4-[8-azanyl-3-[(2~{S})-1-[4-(dimethylamino)butanoyl]pyrrolidin-2-yl]imidazo[1,5-a]pyrazin-1-yl]-~{N}-(1,3-thiazol-2-yl)benzamide 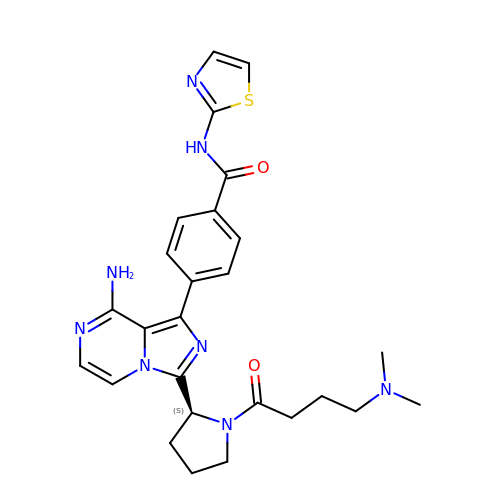| C26 H30 N8 O2 S | HUXVNVAKNWKLJM-IBGZPJMESA-N6-oxime-17-(3-pyridyl)-androst-16-en-3-ol | C24 H32 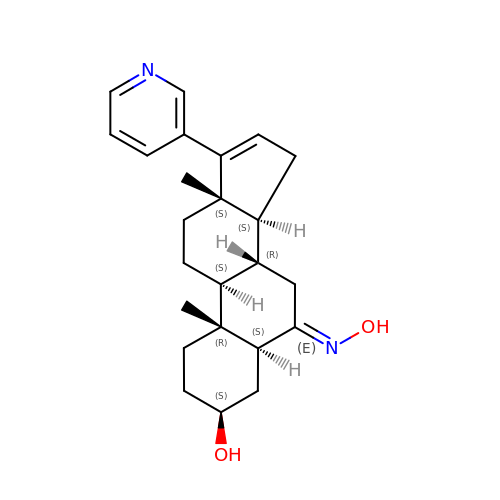N2 O2 | ZKFOPNLIHMQTMV-ZVWUODORSA-N>MGKYQVMKRASEVDLSTVKYKAETMKAPHLTGLSFKLFVNLLEAPLIGSLIVDYLKKDNGMTKIFRNTVIPEEPMFRPEFPSQEPEHDVVIVGEDESPIDRLETALKCLPQYDPSRSLHADPVSSFRYWKIRDYAYAYRSKLTTPLQVAKRIISIIEEFGYDKPPTPFLIRFDANEVIKQAEASTRRFEQGNPISVLDGIFVTIKDDIDCLPHPTNGGTTWLHEDRSVEKDSAVVSKLRSCGAILLGKANMHELGMGTTGNNSNYGTTRNPHDPKRYTGGSSSGSAAIVAAGLCSAALGTDGGGAVRIPSALCGITGLKTTYGRTDMTGSLCEGGTVEIIGPLASSLEDAFLVYAAILGSSSADRYNLKPSP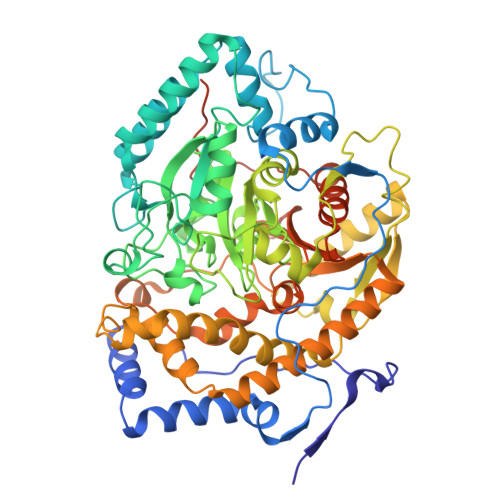PCFPKLLSHNGSNAIGSLRLGKYTKWFNDVSSSDISDKCEDILKLLSNNHGCKVVEIVVPELEEMRAAHVISIGSPTLSSLTPYCEAGKNSKLSYDTRTSFAIFRSFSASDYIAAQCLRRRLMEYHLNIFKDVDVIVTPTTGMTAPVIPPDALKNGETNIQVTTDLMRFVLAANLLGFPAISVPVGYDKEGLPIGLQIMGRPWAEATVLGLAAAVEELAPVTKKPAIFYDILNTNKGEFEAYVEQKLISEEDLNSAVDHHHHHH[12x]Lysenin from the earthworm Eisenia fetida is a pore-forming protein that specifically interacts with sphingomyelin (SM) and may confer innate immunity against parasites by attacking their membranes (Bruhn et al., 2006; Cooper et al., 2001). The structure reveals that lysenin has two domains. The topology of the lysenin structural fold establishes it as a member of the aerolysin family of pore-forming proteins (Szczesny et al., 2011), which appears thus to be conserved from bacteria to annelids. Here we report the crystal structure of lysenin alone, and in complex with the sphingomyelin headgroup phosphocholine (POC), and with SM itself.

The crystal structure of lysenin was first determined in space group P6522, with one molecule per asymmetric unit (a.u.), by multiple isomorphous replacement with anomalous scattering (MIRAS, one SeMet and one Hg derivative) and then in space group P1 with four molecules per a.u. by molecular replacement. The C terminus of lysenin is composed of a β-trefoil motif with a six-stranded antiparallel β-barrel capped on one end by three two-stranded hairpins and a single-turn 310 helix. The five crystallographically independent copies of the molecule (see Experimental Procedures and Table 1), define an ∼45° arc that is subtended by the C-terminal domains hinging at residues 159–168. Residue Gln229 is the gate regulating access to the POC binding pocket: in the apo forms of lysenin, Gln229 is in a closed conformation, blocking the entrance to the POC binding site, but has opened in the POC bound state. Lys185 aids in defining the gate, as it is in a different conformer in the apo form, preventing interaction with the phosphate moiety. The elongated N-terminal domain consists of a 310 helix and 10 β strands, six of which belong to a highly twisted antiparallel β sheet.

>[4x]SAKAAEGYEQIEVDVVAVWKEGYVYENRGSTSVDQKITITKGMKNVNSETRTVTATHSIGSTISTGDAFEIGSVEVSYSHSHEESQVSMTETEVYESKVIEHTITIPPTSKFTRWQLNADVGGADIEYMYLIDEVTPIGGTQSIPQVITSRAKIIVGRQIILGKTEIRIKHAERKEYMTVVSRKSWPAATLGHSKLFKFVLYEDWGGFRIKTLNTMYSGYEYAYSSDQGGIYFDQGTDNPKQRWAINKSLPLRHGDVVTFMNKYFTRSGLCYDDGPATNVYCLDKREDKWILEVVGLVPRGSGHHHHHH> SKSKPDTSAPTSPKVTYKAPVPSGEVYFADSFDRGT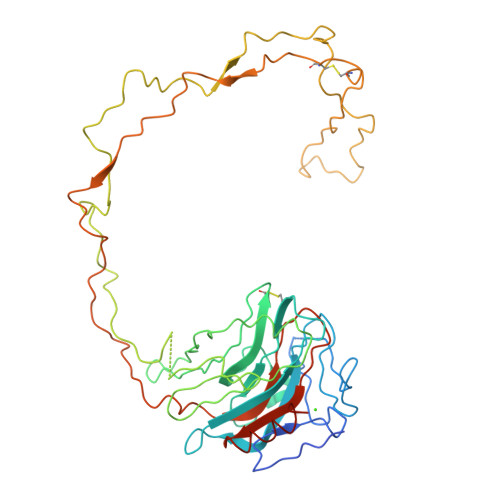LSGWILSKAKKDDTDDEIAKYDGKWEVDEMKETKLPGDKGLVLMSRAKHHAISAKLNKPFLFDTKPLIVQYEVNFQNGIECGGAYVKLLSKTPELNLDQFHDKTPYTIMFGPDKCGEDYKLHFIFRHKNPKTGVYEEKHAKRPDADLKTYFTDKKTHLYTLILNPDNSFEILVDQSIVNSGNLLNDMTPPVNPSREIEDPEDQKPEDWDERPKIPDPDAVKPDDWNEDAPAKIPDEEATKPDGWLDDEPEYVPDPDAEKPEDWDEDMDGEWEAPQIANPKCESAPGCGVWQRPMIDNPNYKGKWKPPMIDNPNYQGIWKPRKIPNPDFFEDLEPFKMTPFSAIGLELWSMTSDIFFDNFIVCGDRRVVDDWANDGWGLKKAADGAAEP> QTQVLFEHPLNEKMRTWLRIEFLIQQLTVNLPIVDHAGALHFFRNVSELLDVFERGEVRTELLKELD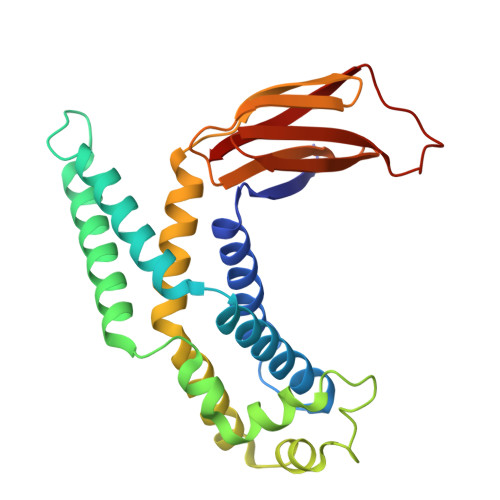RQQRKLQTWIGVPGVDQSRIEALIQQLKAAGSVLISAPRIGQFLREDRLIALVRQRLSIPGGCCSFDLPTLHIWLHLPQAQRDSQVETWIASLNPLTQALTMVLDLIRQSAPFRKQTSLNGFYQDNGGDADLLRLNLSLDSQLYPQISGHKSRFAIRFMPLDSENGQVPERLDFELACC[(2R,3R,4S,5S,6R)-4-formamido-6-methyl-3,5-bis(oxidanyl)oxan-2-yl] [[(2R,3S,5R)-5-[5-methyl-2,4-bis(oxidanylidene)pyrimidin-1-yl]-3-oxidanyl-oxolan-2-yl]methoxy-oxidanyl-phosphoryl] hydrogen phosphate | C17 H27 N3 O15 P2 | 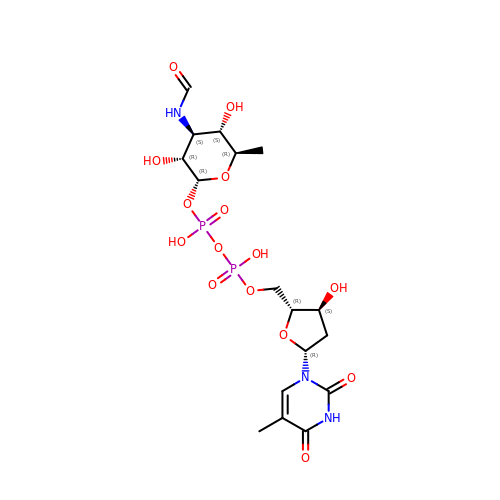XDTNOGIJZRWAPO-ADAYKIPUSA-N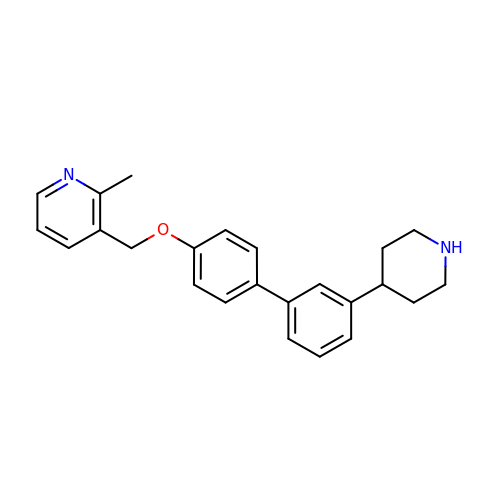2-methyl-3-({[3'-(piperidin-4-yl)[1,1'-biphenyl]-4-yl]oxy}methyl)pyridine | C24 H26 N2 O | ABQOLQKFNLZDIM-UHFFFAOYSA-N>MGSSHHHHHHSSGLEVLFQGPHMESLQQQVAQLLEQQPTLLPAAMAEQLNVTEFDIVHALPEEMVAVVDGSHAQTILESLPEWGPVTTIMTIAGSIFEVKAPFPKGKVARGYYNLMGRDGELHGHLKLENISHVALVSKPFMGRESHYFGFFTAQGENAFKIYLGRDEKRELIPEQ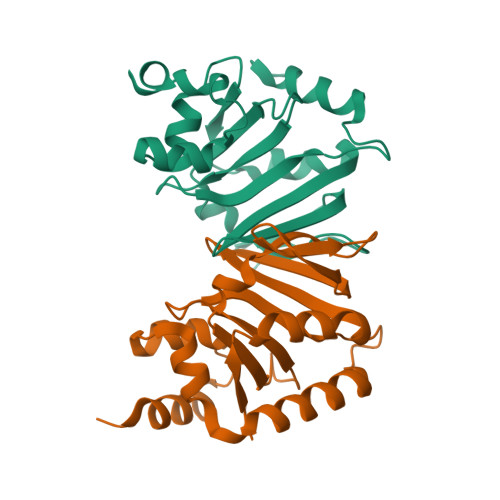VARFKAMQQQHKQ[6x]>[2x]PAPHGGILQDLIARDALKKNELLSEAQSSDILVWNLTPRQLCDIELILNGGFSPLTGFLNENDYSSVVTDSRLADGTLWTIPITLDVDEAFANQIKPDTRIALFQDDEIPIAILTVQDVYKPNKTIEAEKVFRGDPEHPAISYLFNVAGDYYV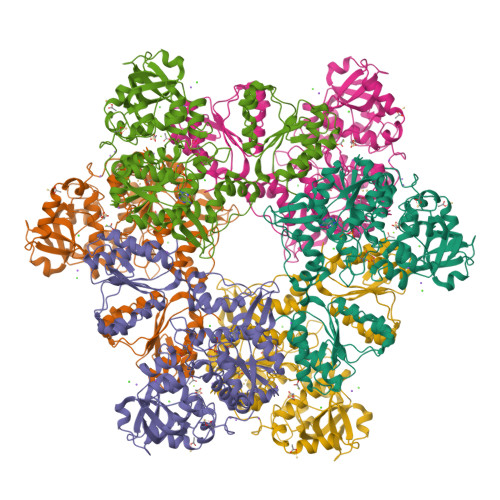GGSLEAIQLPQHYDYPGLRKTPAQLRLEFQSRQWDRVVAFQTRNPMHRAHRELTVRAAREANAKVLIHPVVGLTKPGDIDHHTRVRVYQEIIKRYPNGIAFLSLLPLAMRMSGDREAVWHAIIRKNYGASHFIVGRDHAGPGKNSKGVDFYGPYDAQELVESYKHELDIEVVPFRMVTYLPDEDRYAPIDQIDTTKTRTLNISGTELRRRLRVGGEIPEWFSYPEVVKILRESNPPRPKQGFSIVLGNSLTVSREQLSIALLSTFLQFGGGRYYKIFEHNNKTELLSLIQDFIGSGSGLIIPNQWEDDKDSVVGKQNVYLLDTSSSADIQLESADEPISHIVQKVVLFLEDNGFFVF> MNDIVSAKVLEYKGKKLNFTPEDPAEETIPADELHEHLQKPSTARTKRLKERCRWKHASAGEFIEKSVTAGIERMRYLTEAHKASEGKPEAIRRALGLANVLNKSTLVLQEDEFIVGYHAEDPNMFPLYPELSHMAVQDYLRSDYSPQPADEAAAINEYWKPHSLQSKCQPYFDPADLGRMYQVSSMEAPSFASGYNSIVPPYETVLEDGLLARIKLAEKHIAEAQADMSTFPWNGTKGLDNIAKIDNWKAMVIACKAVISWARRQGRLCKIVAENFETDPKRQAELLEIADICQRIPAEPCKGLKDAMQAKFFTFLICHAIERYASGYAQKEDTLLWPYYKASVVDKKFQPMSHMDAVELVEMERLKISEHGAGKSRAYREIFPGSNDLFILTVGGTNAKGEDACNDMTDAILEAAKRIRTAEPSIVFRYSKKNREKTLRWVFECIRDGLGYPSIKHDEIGTEQMKEYAKFSLNGNGATDEEAHNWVNVLCMSPGIHGRRKTQKTRS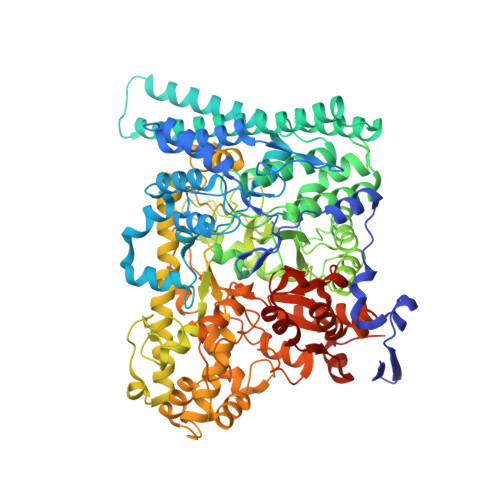EGGGSIFPAKLLEISLNDGYDWSYADMQLGPKTGDLSSLKSFEDVWEAFRKQYQYAINLCISTKDVSRYFEQRFLQMPFVSAIDDGCMELGMDACALSEQPNGWHNPITTIVAANSLVAIKKLVFEEKKYTLEQLSQALKANWEGFEEMRVDFKRAPKWGNDDDYADGIITRFYEEIIGGEMRKITNYSGGPVMPTGQAVGLYMEVGSRTGPTPDGRFGGEAADDGGISPYMGTDKKGPTAVLRSVSKVQKNQKGNLLNQRLSVPIMRSKHGFEIWNSYIKTWHDLNIDHVQFNVVSTDEMRAAQREPEKHHDLIVRVSGYSARFVDIPTYGQNTIIARQEQDFSASDLEFLNVEISGTGSGSSHHHHHH The carboxysome is a natural proteinaceous organelle for carbon fixation in cyanobacteria and chemoautotrophs. It comprises hundreds of protein homologs that self-assemble to form a polyhedral shell structure to sequester cargo enzymes, ribulose 1,5-bisphosphate carboxylase/oxygenase (Rubisco), and carbonic anhydrases. Recent studies have identified the chaperone protein CcmS, which can interact with CcmK1, facilitating β-carboxysome assembly in Syn6803. Here, we determined the structure of the chaperone protein CcmS, which has recently been identified to be involved in β-carboxysome assembly, and its interactions with β-carboxysome proteins.

In the Nos7120 genome, the ccmS gene is located within the gene clusters expressing β-carboxysome proteins and carboxysome-related proteins. ccmS in Nos7120 encodes a protein of 142 amino acids. As determined by SDS-PAGE and Native-PAGE, CcmS functions as a dimer in solution, with the molecular mass of ∼16 kDa for each CcmS monomer. We solved the 1.99 Å crystal structure of the CcmS dimer in space group P212121 by molecular replacement. Two molecules of CcmS form a homodimer in the asymmetric unit, and each CcmS monomer consists of five α-helices and four β-sheets. The two CcmS molecules are rotated symmetrically, with an interaction interface of ∼900 Å2, primarily mediated by hydrogen bonds and salt bridges. Key interactions at the CcmS dimer interface are formed by Arg16-Glu111, Ala109-Gln107, Pro110-Lys104, Asp20-Glu111, and Lys104-Glu111 residues. These residues are highly conserved, suggesting that the dimerization of CcmS is ubiquitous among various β-cyanobacterial species.

>MMFGSTKPESGDSKWRSQLDRFVKENQQDLAALFWGLWLENGDSQGTIGIDLQPTPHFVYCPKDAVEKLNNNVENRLQELLGIIEHNQPEIEVLMIGIGKGEIKLIQFAPEPPPPVCFEQVGKDIDGLLELLEQRMSGEIVV[2x]>GSHMVEIIPVSTTLELRAADESHVPALHQLVLKNKAWLQQSLDWPQYVTSQEETRKHVQGNILLHQRGYAKMYLIFCQNEMAGVLSFNAIEPINKAAYIGYWLDESFQGQGIMSQSLQALMTHYARRGDIRRFVIKCRVDNQASNAVARRNHFTLEGCMKQAEYLNGDYHD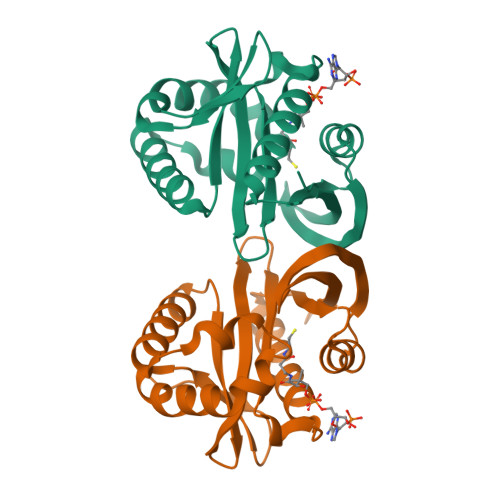VNMYARIIDAD[4x]> SNAMILSQQKYNYLAKVSDSNGVISALAFDQRGALKCLMAQYQMKEPTVAQMEELKVLVSEELTPYASSILLDPEYGLPAAQARDREAGLLLAYEKTGYDANTTSRLPDCLVDWSIKRLKEAGADAVKFLLYYDVDGDPQVNVQKQAYIERIGSECQAEDIPFFLEILTYDETISNNSSVEFAKVKVHKVND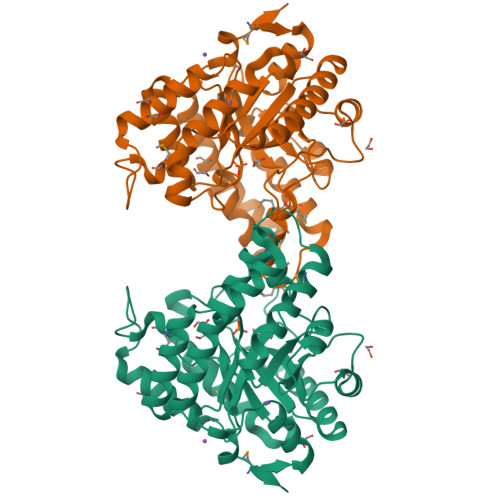AMKVFSAERFGIDVLKVEVPVNMVYVEGFAEGEVVYSKEEAAQAFREQEASTDLPYIYLSAGVSAELFQETLVFAHKAGAKFNGVLCGRATWAGSVQVYMEEGKEAARQWLRTSGLQNINELNKVLKTTASPWTEKVSVG>[3x]MGSSHHHHHHSSGLEVLFQGPHMETAIWIKNSKLPAVLVAAGAFDAAVQALSKQVGVVKLEPLKKYFTNIYEGCRTYIPSTPCELPAQLGYVRAYDDTVSEDQILPYVPGLDVVNEKMNEGYKNFKLNKPDIAIECFREAIYRITLLMVDDAEDEKLAHKILETAREYILG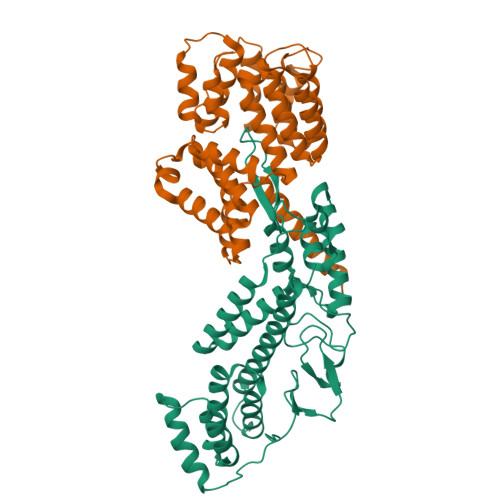LSIELERRSLKEGNTVRMLELAAYFTKAKLSPIHRTNALQVAMSQHFKHKNFLQASYFAGEFLKIISSGPRAEQARKIKNKADSMASDAIPIDFDPYAKFDICAATYKPIYEDTPSVSDPLTGSKYVITEKDKIDRIAMISKIGAPASGLRIRV;>MGSSHHHHHHSQDPMDYFNIKQNYYTGNFVQCLQEIEKFSKVTDNTLLFYKAKTLLALGQYQSQDPTSKLGKVLDLYVQFLDTKNIEELENLLKDKQNSPYELYLLATAQAILGDLDKSLETCVEGIDNDEAEGTTELLLLAIEVALLNNNVSTASTIFDNYTNAIEDTVSGDNEMILNLAESYIKFATNKETATSNFYYYEELSQTFPTWKTQLGLLNLHLQQRNIAEAQGIVELLLSDYYSVEQKENAVLYKPTFLANQITLALMQGLDTEDLTNQLVKLDHEHAFIKHHQEIDAKFDELVRKYDTSN[3x]> MNIFRLTGDLSHLAAIIILLLKIWKSRSCAGISGKSQLLFALVFTTRYLDLFTSFISLYNTSMKLIYIACSYATVYLIYMKFKATYDGNHDTFRVEFLIVPVGGLSFLVNHDFSPLEILWTFSIYLESVAILPQLFMISK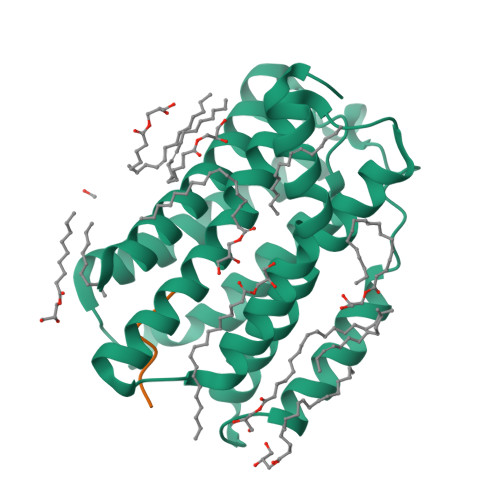TGEAETITTHYLFFLGLYRALYLVNWIWRYYFEGFFDLIAVVAGVVQTVLYCDFFYLYVTKVLKGKK;> AEKDEL> MPLAFCGTENHSAAYRVDQGVLNNGCFVDALNVVPHVFLLFITFPILFIGWGSQSSKVHIHHSTWLHFPGHNLRWILTFILLFVLVCEIAEGILSDGVTESRHLHLYMPAGMAFMAAITSVVYYHNIETSNFPKLLIALLIYWTLAFITKTIKFVKFYDHAIGFSQLRFCLTGLLVILYGMLLLVEVNVIRVRRYIFFKTPREVKPPEDLQDLGVRFLQPFVNLLSKGTYWWMNAFIKTAHKKPIDLRAIAKLPIAMRALTNYQRLCVAFDAQARKDTQSPQGARAIWRALCHAFGRRLILSSTFRILADLLGFAGPLCIFGIVDHLGKENHVFQPKTQFLGVYFVSSQEFLGNAYVLAVLLFLALLLQRTFLQASYYVAIETGINLRGAIQTKIYNKIMHMSTSNLSMGEMTAGQICNLVAIDTNQLMWFFFLCPNLWTMPVQIIVGVILLYYILGVSALIGAAVIILLAPVQYFVATKLSQAQRTTLEHSNERLKQTNEMLRGMKLLKLYAWESIFCSRVEVTRRKEMTSLRAFAVYTSISIFMNTAIPIAAVLITFVGHVSFFKESDLSPSVAFASLSLFHILVTPLFLLSSVVRSTVKALVSVQKLSEFLSSAEIREEQCAPREPAPQGQAGKYQAVPLKVVNRKRPAREEVRDLLGPLQRLAPSMDGDADNFCVQIIGGFFTWTPDGIPTLSNITIRIPRGQLTMIVGQVGCGKSSLLLATLGEMQKVSGAVFWNSNLPDSEGEDPSSPERETAAGSDIRSRGPVAYASQKPWLLNATVEENITFESPFNKQRYKMVIEACSLQPDIDILPHGDQTQIGERGINLSGGQRQRISVARALYQQTNVVFLDDPFSALDVHLSDHLMQAGILELLRDDKRTVVLVTHKLQYLPHADWIIAMKDGTIQREGTLKDFQRSECQLFEHWKTLMNRQDQELEKETVMERKASEPSQGLPRAMSSRDGLLLDEEEEEEEAAESEEDDNLSSVLHQRAKIPWRACTKYLSSAGIL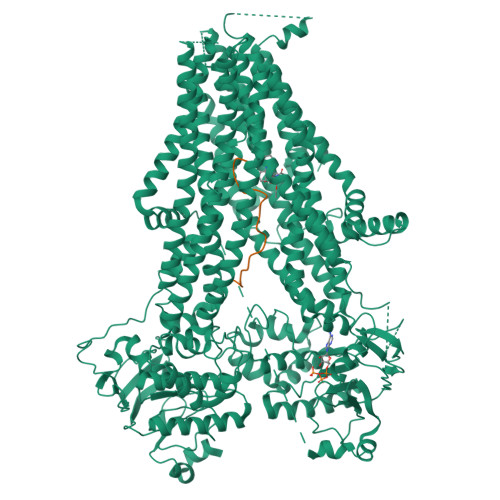LLSLLVFSQLLKHMVLVAIDYWLAKWTDSALVLSPAARNCSLSQECDLDQSVYAMVFTLLCSLGIVLCLVTSVTVEWTGLKVAKRLHRSLLNRIILAPMRFFETTPLGSILNRFSSDCNTIDQHIPSTLECLSRSTLLCVSALTVISYVTPVFLVALLPLAVVCYFIQKYFRVASRDLQQLDDTTQLPLVSHFAETVEGLTTIRAFRYEARFQQKLLEYTDSNNIASLFLTAANRWLEVCMEYIGACVVLIAAATSISNSLHRELSAGLVGLGLTYALMVSNYLNWMVRNLADMEIQLGAVKRIHALLKTEAESYEGLLAPSLIPKNWPDQGKIQIQNLSVRYDSSLKPVLKHVNTLISPGQKIGICGRTGSGKSSFSLAFFRMVDMFEGRIIIDGIDIAKLPLHTLRSRLSIILQDPVLFSGTIRFNLDPEKKCSDSTLWEALEIAQLKLVVKALPGGLDAIITEGGENFSQGQRQLFCLARAFVRKTSIFIMDEATASIDMATENILQKVVMTAFADRTVVTIAHRVHTILSADLVMVLKRGAILEFDKPETLLSQKDSVFASFVRADK;> MLSRKGIIPEEYVLTRLAEDPTEPRYRTRERRARFVSKKGNCNVAHKNIREQGRFLQDVFTTLVDLKWPHTLLIFTMSFLCSWLLFAMVWWLIAFAHGDLAPGEGTNVPCVTSIHSFSSAFLFSIEVQVTIGFGGRMVTEECPLAILILIVQNIVGLMINAIMLGCIFMKTAQAHRRAETLIFSKHAVITPRHGRLCFMLRVGDLRKSMIISATIHMQVVRKTTSPEGEVVPLHQVDIPMENGVGGNSIFLVAPLIIYHVIDSNSPLYDLAPSDLHHHQDLEIIVILEGVVETTGITTQARTSYLADEILWGQRFVPIVAEEDGRYSVDYSKFGNTVKVPTPLCTARQLDEDRSLLDALTLASSRGPLRKRSVAVAKAKPKFSISPDSLS>[2x]MATEPKAGRPSDYMPEVADDICSL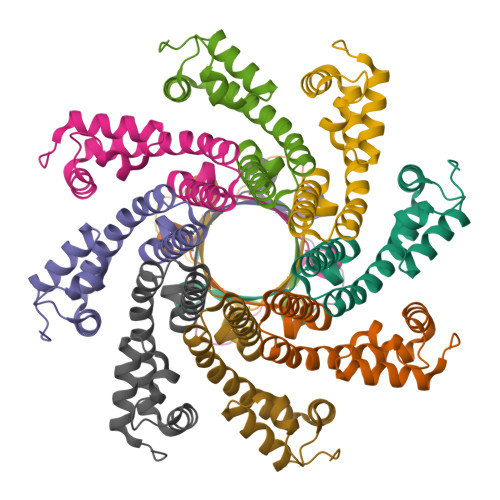LSSGESLLKVCKRPGMPDKSTVFRWLAKHEDFRDEYAKATEARADSIFEEIFEIADNAIPDAAEVAKARLRVDTRKWALARMNPRKYGDKVTNELVGKDGGAIQIETSPMSTLFGK> MDQECIENYAKVNGIYIYYKLCKAPEEKAKLMTMHGGPGMSHDYLLSLRDMTKEGITVLFYDQFGCGRSEEPDQSKF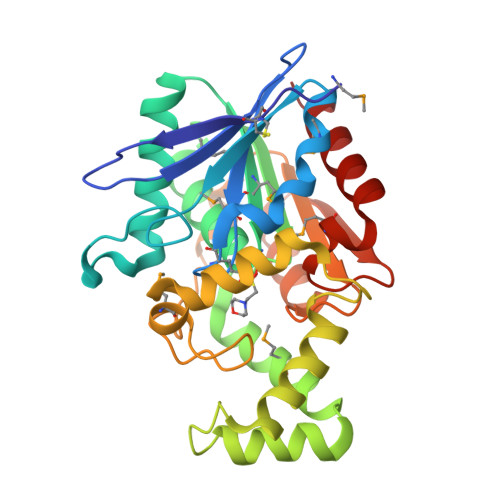TIDYGVEEAEALRSKLFGNEKVFLMGSSYGGALALAYAVKYQDHLKGLIVSGGLSSVPLTVKEMNRLIDELPAKYRDAIKKYGSSGSYENPEYQEAVNYFYHQHLLRSEDWPPEVLKSLEYAERRNVYRIMNGPNEFTITGTIKDWDITDKISAIKIPTLITVGEYDEVTPNVARVIHEKIAGSELHVFRDCSHLTMWEDREGYNKLLSDFILKHL> MGSHHHHHHHHHSGHMMAAAVASLATLAAEPREDAFRKLFRFYRQSRPGTADLGAVIDFSEAHLARSPKPGVPQVVRFPLNVSSVTERDAERVGLEPVSKWRAYGLEGYPGFIFIPNPFLPGCQRHWVKQCLKLYS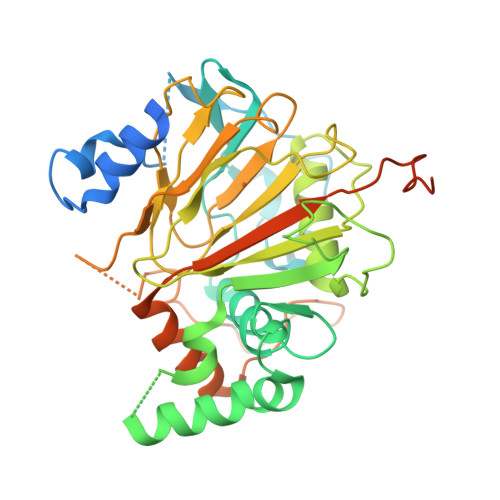QKPNVCNLDKHMTKEETQGLWEQSKEVLRSKEVTKRRPRSLLERLRWVTLGYHYNWDSKKYSADHYTPFPSDLAFLSEQVATACGFQGFQAEAGILNYYRLDSTLGIHVDRSELDHSKPLLSFSFGQSAIFLLGGLKRDEAPTAMFMHSGDIMVMSGFSRLLNHAVPRVLPHPDGECLPHCLETPLPAVLPSNSLVEPCSVEDWQVCATYLRTARVNMTVRQVLATGQDFPLEPVEETKRDIAADGLCHLHDPNSPVKRKRLNPNS> MNDWASLGIGSIGEAVFSKLLKVVIDEAKKFKAFKPLSKDLVSTMEILFPLTQKIDSMQKELDFGVKELKELRDTIERADVAVRKFPRVKWYEKSKYTRKIERINKDMLKFCQIDLQLLQHRNQLTLLGLTGNEVNSVDGLSKRMDLLSVPAPVFRDLCSVPKLDKVIVGLDWPLGELKKRLLDDSVVTLVVSAPPGCGKTTLVSRLCDDPDIKGKFKHIFFNVVSNTPNFRVIVQNLLQHNGYNALTFENDSQAEVGLRKLLEEL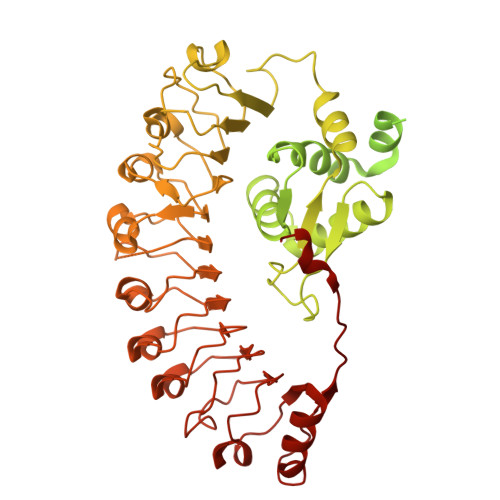KENGPILLVLDDVWRGADSFLQKFQIKLPNYKILVTSRFDFPSFDSNYRLKPLEDDDARALLIHWASRPCNTSPDEYEDLLQKILKRCNGFPIVIEVVGVSLKGRSLNTWKGQVESWSEGEKILGKPYPTVLECLQPSFDALDPNLKECFLDMGSFLEDQKIRASVIIDMWVELYGKGSSILYMYLEDLASQNLLKLVPLGTNEHEDGFYNDFLVTQHDILRELAICQSEFKENLERKRLNLEILENTFPDWCLNTINASLLSISTDDLFSSKWLEMDCPNVEALVLNLSSSDYALPSFISGMKKLKVLTITNHGFYPARLSNFSCLSSLPNLKRIRLEKVSITLLDIPQLQLSSLKKLSLVMCSFGEVFYDTEDIVVSNALSKLQEIDIDYCYDLDELPYWISEIVSLKTLSITNCNKLSQLPEAIGNLSRLEVLRLCSSMNLSELPEATEGLSNLRFLDISHCLGLRKLPQEIGKLQNLKKISMRKCSGCELPESVTNLENLEVKCDEETGLLWERLKPKMRNLRVQEEEIEHNLNLLQMF N-{[2-(1,3-dimethyl-2-oxo-6-sulfanylidene-1,2,3,6-tetrahydro-7H-purin-7-yl)ethyl]carbamoyl}methanesulfonamide 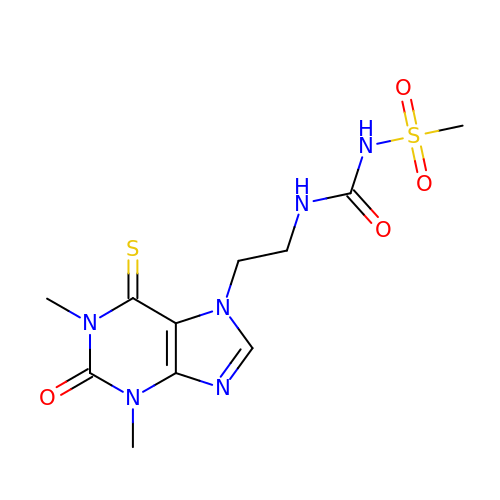| C11 H16 N6 O4 S2 | CEDCEGLXBVDTJP-UHFFFAOYSA-N>[6x]GMSKRANKLVIVTEKVLLKKVAKIIEEAGATG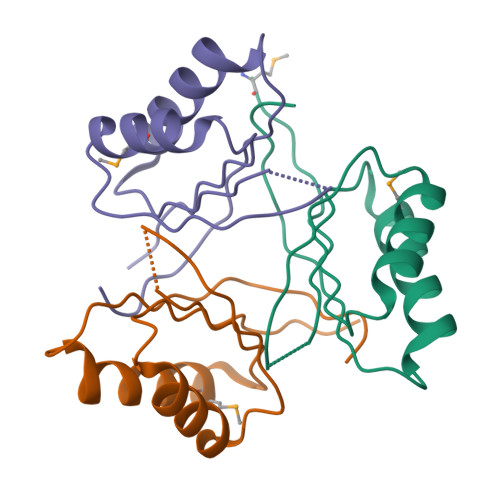YTVVDTGGKGSRNVRSTGKPNTSDTDSNVKFEVLTENREMAEKIADQVAIKFFTDYAGIIYICEAEVLYGRTFCGPDGC By using a flavin transferase and carving a flavinylation motif in target proteins, we demonstrate that “dissociable” flavoproteins can be turned into covalent flavoproteins. Specifically, four different flavin mononucleotide-containing proteins were engineered to undergo covalent flavinylation: a light-oxygen-voltage domain protein, a mini singlet oxygen generator, a nitroreductase, and an old yellow enzyme-type ene reductase. The crystal structures of the designed covalent flavoproteins confirmed the designed threonyl-phosphate linkage. The elucidated crystal structures confirm that the covalent attachment does not significantly perturb the binding and microenvironment of the redox active part of the flavin cofactor.

We recently discovered a novel BtNR that is capable of reducing a variety of nitro compounds. Inspection of the crystal structure of BtNR revealed three potential sites for flavinylation: three neighboring residues that are positioned close to the FMN phosphate (R15, H16, and A17). The dimeric BtNR-F3 structure was determined to be 2.0 Å. Rms deviation with the structure of BtNR wt is 0.5 Å. The mutated residues from BtNR wt 11AYNFRHA17 to BtNR-F3 11DGLSGAT17 represent the flavin fix site. Intriguingly, for the first 15 residues of both chains, including Asp11, no electron density was observed, and these residues are probably flexible. The FMN phosphate group shifts 1.6 Å toward OG1 of Thr17, to which it is covalently attached. Despite the Cα atom of Thr17 shifting by 2.7 Å compared to that of wt Ala17, the covalent bond is formed. The phosphate group in BtNR wt is stabilized by the side chains of Arg15, Lys209, and Arg211 and the backbone nitrogen of Ala17. In BtNR-F3, besides the covalent linkage to Thr17, the interaction with R211 remains.

>[2x]MADVKKQILDDGLSGATTKEFDPNKKVSDSDFEFILETGRLSPSSLGLEPWKFVVVQNPEFREKLREYTWGAQKQLPTASHFVLILARTAKDIKYNADYIKRHLKEVKQMPQDVSEGYISKTEEFQKNDLHLLESDRTLFDWASKQTYIALGNMMTAAAQIGVDSCPIEGFQYDHIHRILEEEGLLENGSFDISVMAAFGYRVRDPRPKTRSAVEDVVKWV>[2x]DPMFIIVCYDVETITQEGRARLRKVAKTCESHGQRVQKSVFECQLEPADYLQFEAKLSKIINSKTDNLRIYSLDAISVSKIKQFGVSNILDF

The genome of pathogenic Leptospira interrogans serovars (Copenhageni and Lai) are predicted to have CRISPR-Cas of subtypes I-B and I-C. Cas2, one of the core Cas proteins, has a crucial role in adaptive defense against foreign nucleic acids. The Cas2 proteins (80–120 residues) are core metallonucleases found universally in all CRISPR-bearing taxa. In Leptospira, the CRISPR-Cas subtype I-C lacks the CRISPR array component and is thus considered an orphan CRISPR-Cas system. Unlike Cas2 from other organisms, the purified rLinCas2C and rLinCas2C_Lai exhibited metal-dependent DNase and metal-independent RNase activity.

The crystal structure of rLinCas2C obtained at the resolution of 2.60 Å revealed the protein is in apostate conformation and contains N- (1–71 amino acids) and C-terminal (72–90 amino acids) regions, with the former possessing a ferredoxin fold. The crystal structure of rLinCas2C encloses the signature N-terminal ferredoxin domain (βαββαβ). LinCas2C crystal is composed of a total of three α-helices (α1–α3) and five anti-parallel β-strands (β1–β5) for the Cas2 orthologs enlisted in Table 2. In rLinCas2C, upon dimerization, the buried surface area is 3,430 Å2, identified by PDBePISA. A total of 33 hydrogen bonds were formed between two protomers of LinCas2C as analyzed by Coot. The rLinCas2C dimer demonstrates that the β5 strand (6 residues) of one protomer bridges with the β4 strand (5 residues) of another protomer by 8–10 hydrogen bonds and several other residues enlisted in Supplementary Table S2. The crystal structure of rLinCas2C (dimeric form) indicates it is in a catalytically inactive conformational state as the distance between the conserved Asp8 residue of each protomer is 11.0 Å (as opposed to 6.5 Å in SsoCas2). The distance of 11.0 Å seems too far to coordinate a single Mg2+ ion of the protein. For these aspartates to bind a bridging metal, the rLinCas2C would need to undergo either a major conformational change of the β1 or ferredoxin fold region or altogether the dimer orientation. The mapping of the surface electrostatic potential of rLinCas2C demonstrated the presence of a positive charge at the putative nucleic acid substrate-binding loop (L1 and L2) and the α1 region. In LinCas2C, alanine replacement mutation of conserved residues Tyr7, Asp8, Arg33, and Phe39 and loop L2 abolishes DNase activity, whereas moderate reduction of RNase activity was evident in selected mutants.> MSDFNLVGVIRVMPTD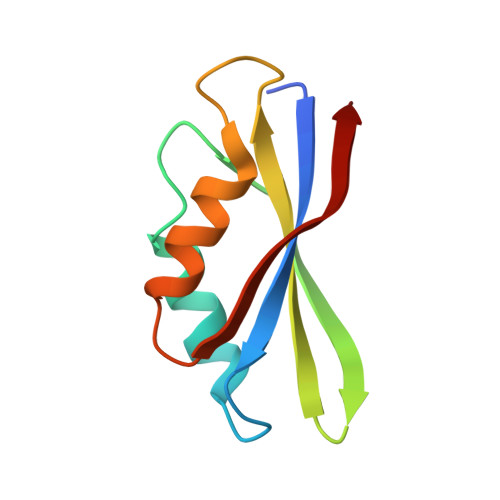PDVNLDELEEKLKKVIPEKYGLAKVEREPIAFGLVALKFYVLGRDEEGYSFDEVAEKFEEVENVESAEVETVSRI> ITSNPDEEWREVRHTGLVQKLIVYPPPPTKGGLGVTNEDLECLEEGEFLNDVIIDFYLKYLILEKASDELVERSHIFSSFFYKCLTRKENNLTEDNPNLSMAQRRHKRVRTWTRHINIFNKDYIFVPVNESSHWYLAVICFPWLEEAVYEDFPQTVSQQ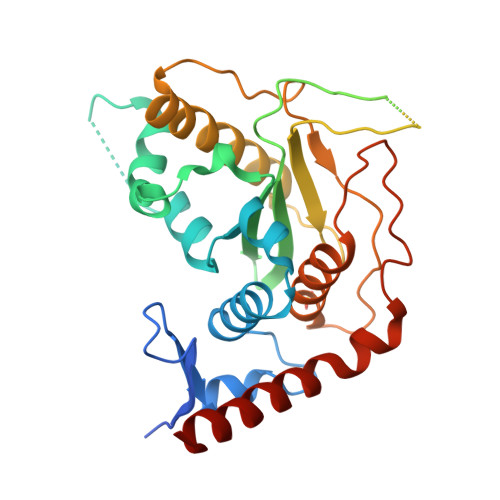SQAQQSQNDNKTIDNDLRTTSTLSLSAEDSQSTESNMSVPKKMCKRPCILILDSLKAASVQNTVQNLREYLEVEWEVKLKTHRQFSKTNMVDLCPKVPKQDNSSDCGVYLLQYVESFFKDPIVNFELPIHLEKWFPRHVIKTKREDIRELILKLHLQQQKGSSS>[2x]GSVFWEPLSYFNPSTWEKADGYSNGGVFNCTWRANNVNF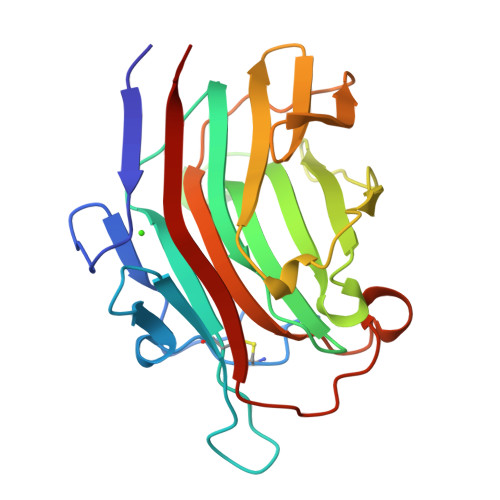TNDGKLKLGLTSSAYNKFDCAEYRSTNIYGYGLYEVSMKPAKNTGIVSSFFTYTGPAHGTQWDEIDIEFLGKDTTKVQFNYYTNGVGGHEKVISLGFDASKGFHTYAFDWQPGYIKWYVDGVLKHTATANIPSTPGKIMMNLWNGTGVDDWLGSYNGANPLYAEYDWVKYTSN>[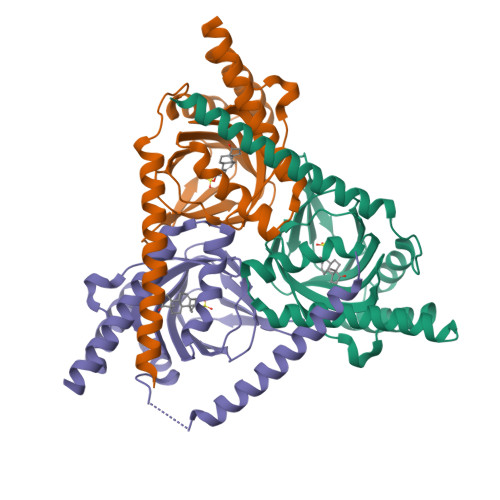6x]GGGGRSVDTMALWLGLRAVLVVAGLAVLLQLIRGWLSSKSYVFNREEIARLAKEHSGLDYEVAFSKIIVELRKKHPGHILQDEDLQWVFVNAGGWMGSMCLLHASLTEYVLLFGTAVDTGGHSGRYWAEISDTILSGTFRQWKEGTTKSEIFYPGDTIVHEVGEATSVQWSSGTWMVEYGRGFIPSTLAFALADTIFSTQDFLTLFYTVKVYSKALLLEASTHLSQLGFFAAA> MGMVVALGLDFGTSGARAIACDFDSDRSVSVSVTFPKTSQNWPQVWREALWQLLTQIPADWRSRIERIAIDGTSGTVLLCDREGQPQTEPLLYNQACPIDLADLADWVPADHAALSSTSSLAKLWFWQQQFGALPPDWQILAQADWLSLQLHGCSQQSDYHNALKLGYSPDRERFSKNLLDSELGALLPVVHEPGVAIGPILPAIAQE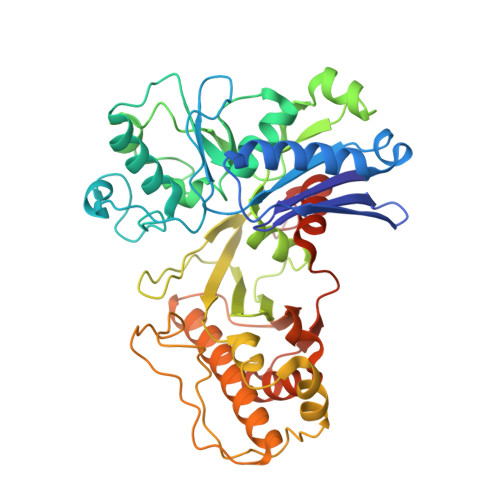FGLSPDCQICAGTTASIAAFLASGAHQPGEAVTSLGSTIVLKLLSQVAVSDRLTGVYSHKLGGYWLTGGASNCGGATLRQFFPDTELESLSCQIDPTKKSGLDYYPLPSRGERFPIADPDRLPQLEPRPENPVQFLQGLLEGLTQVETLGYQRLQDLGATPLKRIWTAGGGAKNAVWQQLRQQAIGVPIAIAPNTEAAFGTARLAAFGLAAFHSAGLKRTLEHHHHHH> GPTVEEAKAEKET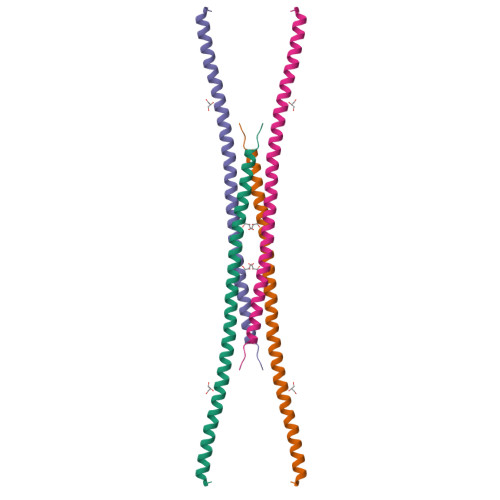ELSLQKEQLQLKIIEIEDDVEKWQKEKDRIKSFTTNEKAILEQNFRDLVRELEKQKEEVRAALEQREQDAVDQVKVIVD5'-O-[(S)-hydroxy(octanoyloxy)phosphoryl]adenosine | C18 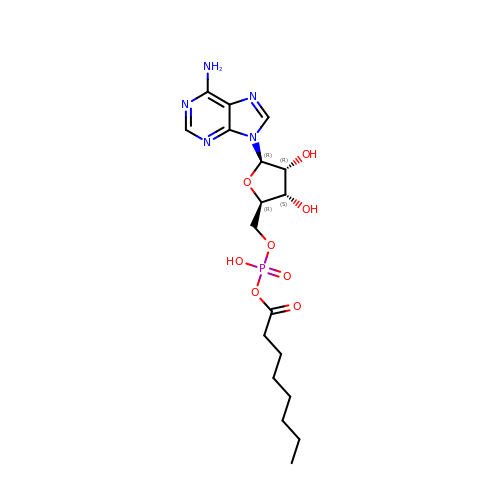H28 N5 O8 P | AJYSFZDSJUTHRW-XKLVTHTNSA-N>MPLSRVEELVADIRAGKMVILMDDEDRENEGDLVIAATHVRPEDINFMITHARGLVCLTLSRERCKQLNLPLMVDQNGAQHGTNFTLSIEAAEGITTGISAAERAHTIQAAVAAHAKPTDIVQPGHIFPLMAQPGGVLHRAGHTEAGCDLARLAGLEPASVICEIIKEDGTMARRADLEIFAEKHGLKIGTIADLIHYRMTNEQTVERLDQRTIQTEYGSFELYRYREIGNPDIHLALVKGEPKEGVTTVRVHGFSPVRDLLKLNKADGEPAWNLDRALQTIAASDRGVLVWIGQDHLQDLGPALDDLTKPKPVKSNAAL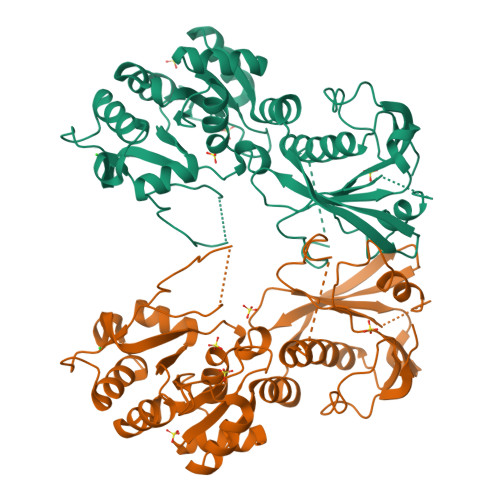SHQYQTIGVGAQILRDLGVEKMKLLSSPLRFNALSGFNLEVVEYVTADQITTK[2x]>THWFHRNPLKATAPVSFNYYGVVTGPSASKICNDLRSSRARLLELFTDLSCNPEMMKNAADSYFSLLQGFINSLDESTQESKLRYIQNFKWTDTLQGQVPSAQQDAVFELISMGFNVALWYTKYASRLAGKENITEDEAKEVHRSLKIAAGIFKHLKESHLPKLITPAEKGRDLESRLIEAYVIQCQAEAQEVTIARAIELKHAPGLIAALAYETANFYQKADHTLSSLEPAYSAKWRKYLHLKMCFYTAYAYCYHGETLLASDKCGEAIRSLQEAEKLYAKAEALCKEYGETKGPGPTVKPSGHLFFRKLGNLVKNTLEKCQRENGFIYFQKIPTEAPQLELKANYGLVEPIPFEFPPTSVQWTP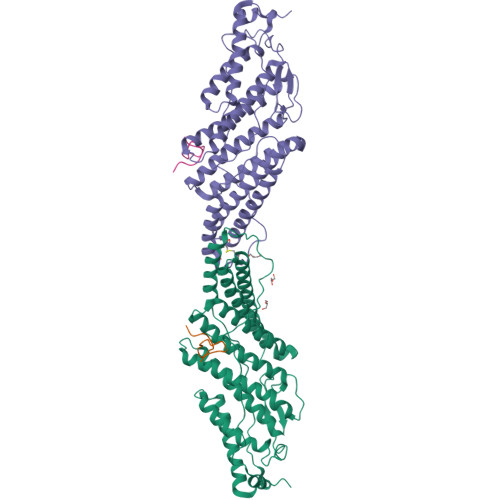ETLAAFDLTK[2x];>TKNKDGVLVDEFGLPQIPAS[2x]> MAMSNGNNDFVVLSNSSIATSAANPSPLTPCDGDHAAQQLTPKEATRTKVSPNGCLQLNGTVKSSFLPLDNQRMPQMLPQCCHPCPYHHPLTSHSSHQECHPEAGPAAPSALASCCMQPHSEYSASLCPNHSPVYQTTCCLQPSPSFCLHHPWPDHFQHQPVQQHIANIRPSRPFKLPKSYAALIADWPVVVLGMCTMFIVVCALVGVLVPELPDFSDPLLGFEPRGTAIGQRLVTWNNMVKNTGYKATLANYPFKYADEQASSLEVLFQGPGSEVDWNFHKDSFFCDVPSDRYSRVVFTSSGGETLWNLPAIKSMCNVDNSRIRSHPQFGDLCQRTTAASCCPSWTLGNYIAILNNRSSCQKIVERDVSHTLKLLRTCAKHYQNGTLGPDCWDMAARRKDQLKCTNVPRKCTKYNAVYQILHYLVDKDFMTPKTADYATPALKYSMLFSPTEKGESMMNIYLDNFENWNSSDGVTTITGIEFGIKHSLFQDYLLMDTVYPAIAIVIVLLVMCVYTKSMFITLMTMFAIISSLIVSYFLYRVVFHFEFFPFMNLTALIILVGIGANNAFVLCDVWNYTKFDKPHAETSETVSITLQHAALSMFVTSFTTAAAFYANYVSNITAIRCFGVYAGTAILVNYVLMVTWLPAVVVLHERYLLNIFTCFKKPQQQIYDNKSCWTVACQKCHKVLFAISEASRIFFEKVLPCIVIKFRYLWLFWFLALTVGGAYIVCIN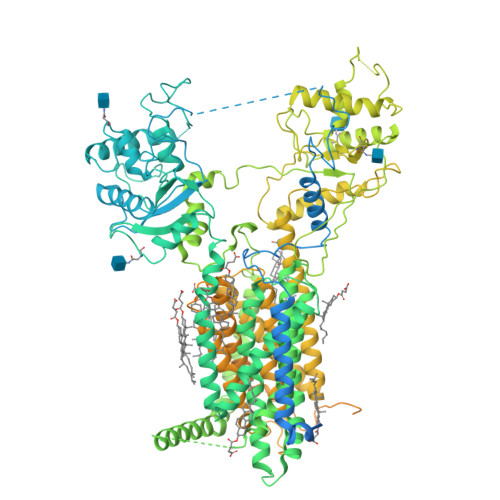PKMKLPSLELSEFQVFRSSHPFERYDAEYKKLFMFERVHHGEELHMPITVIWGVSPEDNGNPLNPKSKGKLTLDSSFNIASPASQAWILHFCQKLRNQTFFYQTDEQDFTSCFIETFKQWMENQDCDEPALYPCCSHWSFPYKQEIFELCIKRAIMELERSTGYHLDSKTPGPRFDINDTIRAVVLEFQSTYLFTLAYEKMHQFYKEVDSWISSELSSAPEGLSNGWFVSNLEFYDLQDSLSDGTLIAMGLSVAVAFSVMLLTTWNIIISLYAIISIAGTIFVTVGSLVLLGWELNVLESVTISVAVGLSVNFAVHYGVAYRLAPDPDREGKVIFSLSRVGSAMAMAALTTFVAGAMMMPSTVLAYTQLGTFMMLIMCISWAFATFFFQCMCRCLGPQGTCGQIPLPKKLQCSAFSHALSTSPSDKGQSKTHTINAYHLDPRGPKSELEHEFYELEPLASHSCTAPEKTTYEETHICSEFFNSQAKNLGMPVHAAYNSELSKSTESDAGSALLQPPLEQHTVCHFFSLNQRCSCPDAYKHLNYGPHSCQQMGDCLCHQCSPTTSSFVQIQNGVAPLKATHQAVEGFVHPITHIHHCPCLQGRVKPAGMQNSLPRNFFLHPVQHIQAQEKIGKTNVHSLQRSIEEHLPKMAEPSSFVCRSTGSLLKTCCDPENKQRELCKNRDVSNLESSGGTENKAGGKVELSLSQTDASVNSEHFNQNEPKVLFNHLMGEAGCRSCPNNSQSCGRIVRVKCNSVDCQMPNMEANVPAVLTHSELSGESLLIKTL> MNLEMLESQPLPEIVTLREE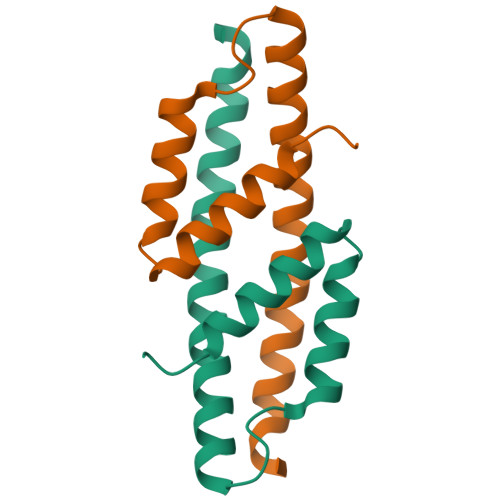IDRLDAEILALVKRRAEVSQAIGKARMASGGPRLDHSREMKIIERYSELGPVGKDLAILLLRLGRGPDAM3-(4-{[(2-chlorophenyl)carbamoyl]amino}-1H-pyrazol-1-yl)-N-(2-methylpyridin-4-yl)benzamide | C23 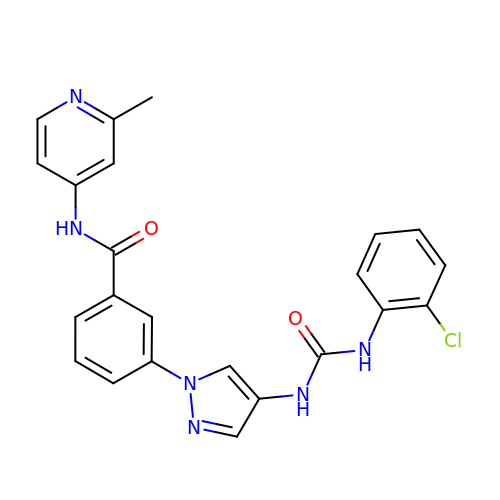H19 Cl N6 O2 | XMZFQCOWVFCHQO-UHFFFAOYSA-N> MHHHHHHSPALPAFLLCSTLLVIKMYVVAIITGQVRLRKKAFANPEDALRHGGPQYCRSDPDVERCLRAHRNDMETIYPFLFLGFVYSFLGPNPFVAWMHFLVFLVGRVAHTVAYLGKLRAPIRSVTY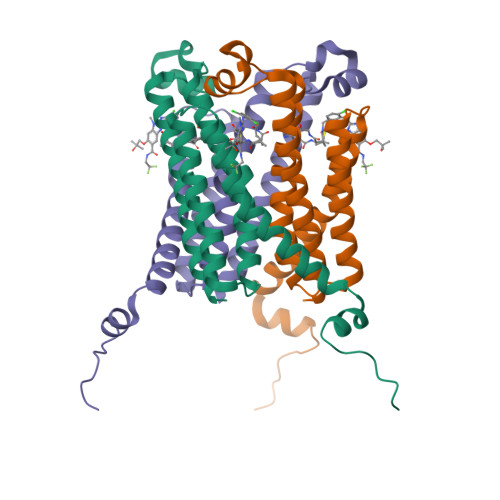TLAQLPCASMALQILWEAARHFLPAALRAALLGRLRTLRPWADYKDDDDK FAD-MDL72527 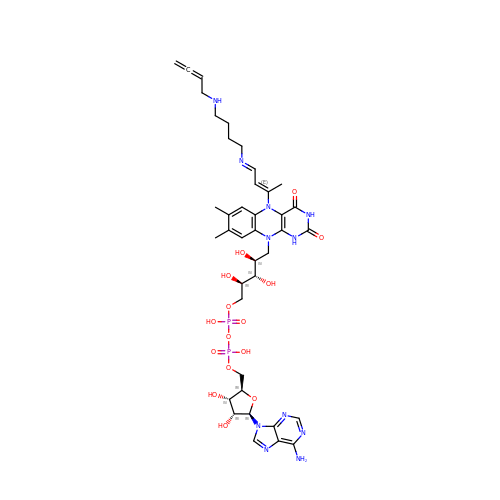adduct | C39 H53 N11 O15 P2 | DOENOACRUGDSKX-BYAUSPTGSA-N Myo inositol 3,4,5,6 tetrakisphosphate | C6 H16 O18 P4 | 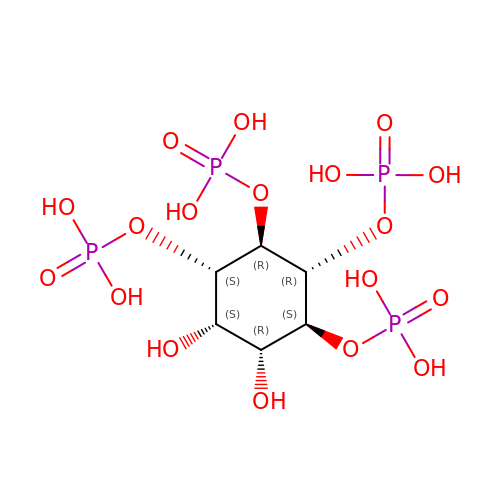MRVYFOANPDTYBY-UZAAGFTCSA-N Lytic Polysaccharide Monooxygenases (LPMOs) are a recently discovered group of copper metalloenzymes that depolymerize recalcitrant polysaccharides like lignocellulose and chitin by oxidative cleavage of the glycosidic bonds. The His-brace is made up of the Cu metal center coordinated with the imidazole ring Nδ1 and backbone N atoms of the terminal His and the imidazole ring nitrogen Nε2 atom of a His located later in the protein sequence. In this study, the focus is on AA9 LPMOs, where a conserved His and Gln (His147 and Gln162 in LsAA9A) form the 2nd coordination sphere and a strong H-bonding network has been shown in the crystal structures. Our results reveal that the conserved His residue of the 2nd coordination sphere in AA9 LPMOs is generally singly protonated.

Three structures of AA9 from LsAA9A and Thermoascus aurantiacus (TaAA9A) were determined in this study. Three out of the six high resolution AA9A structures, two from Lentinus similis (two different data sets for the same enzyme) and one from Thermoascus aurantiacus, were determined in this study. The data for all the three structures extends to very high resolutions. In TaAA9A, the completeness of the data cutting at resolutions of 1.06 Å and 1.2 Å are 40.4% and 94.6%, respectively. Thus, all three datasets have good completeness beyond the threshold of 1.2 Å considered necessary for partial unrestrained refined, and therefore, we decided to extend the datasets to include higher resolutions, which can still contribute to improving the data/parameter ratio in refinement. His147 in LsAA9A and His164 in TaAA9A were investigated for the protonation states at Nδ1 and Nε2 atoms of the imidazole ring of the histidines. Here, the His residues (of the primary and secondary coordination spheres) undergo unrestrained refinement, while the residues in the rest of the structure undergo restrained refinement. Our results suggest that the His of the secondary co-ordination sphere is singly protonated at the Nε2 atom in most if not all structures. Examination of the micro-environment of this His residue in all the LPMO structures of this study show also that the distance of the Nδ1 atom from main chain N-H is between 2.75 to 2.95 Å. Therefore, this N is likely to serve as a H-bond acceptor and reinforcing the view that the His is unlikely to be doubly protonated.

>HGFVQNIVIDGKNYGGYLVNQYPYMSNPPEVIAWSTTATDLGFVDGTGYQTPDIICHRGAKPGALTAPVSPGGTVELQWTPWPDSHHGPVINYLAPCNGDCSTVDKTQLEFFKIAESGLINDDNPPGIWASDNLIAANNSWTVTIPTTIAPGNYVLRHEIIALHSAQNQDGAQNYPQCINLQVTGGGSDNPAGTLGTALYHDTDPGILINIYQKLSSYIIPGPPLYTG[2x]>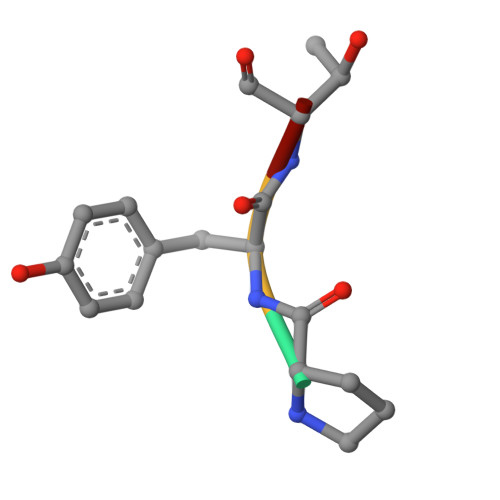 PYTV> MGSDKIHHHHHHENLYFQGMNTIDIAKSYITAIQTGDHATLGSIISPDVIWHQPGNHQFSGTHRGMAVVGPMLGKMMEVSNGTFAISRADDYMASGDWVAITLEFSGQANGVTLKQAGVDLLRIEDGKIVEVRLFSADQT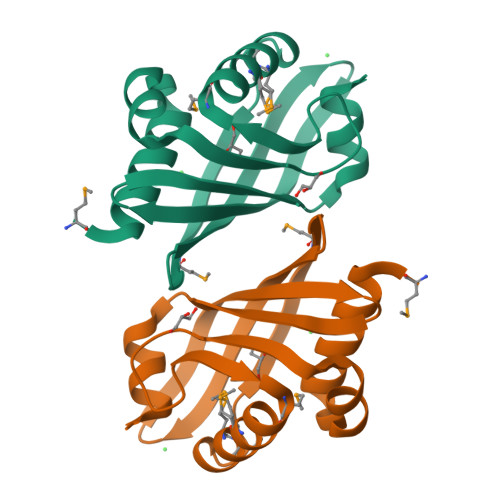QEDAFWGR> GAMADTCMSRIVKEY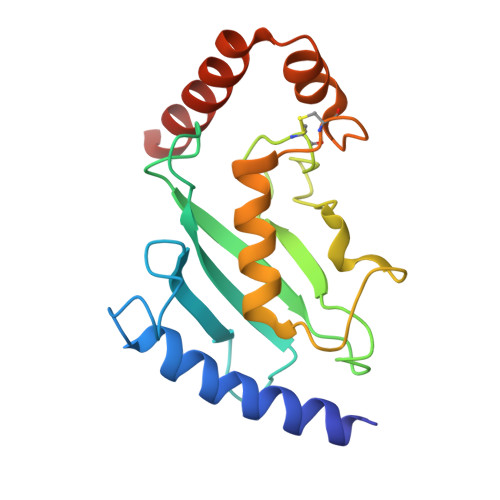KVILKTLASDDPIANPYRGIIESLNPIDETDLSKWEAIISGPSDTPYENHQFRILIEVPSSYPMNPPKISFMQNNILHCNVKSATGEICLNILKPEEWTPVWDLLHCVHAVWRLLREPVCDSPLDVDIGNIIRCGDMSAYQGIVKYFLAERERINNH Cellular responses to replication-associated DNA damage are centred around Proliferating Cell Nuclear Antigen (PCNA), a DNA clamp that acts as a processivity factor for eukaryotic DNA polymerases. Structurally, ZRANB3 belongs to the Sucrose Non-Fermenting 2 (SNF2) family of ATPases and contains several identifiable domains and motifs, which provide specificity for a number of defined substrates. These include the amino-terminal SNF2 ATPase core, two PCNA binding motifs (the PIP box and the APIM motif), a specific type of zinc-finger (Npl4 Zinc-Finger, NZF) and the HNH nuclease domain (named after the three most conserved residues). We have previously identified ZRANB3 as a structure-specific endonuclease that plays a role in the replication stress response. We further defined PCNA as a key regulator of ZRANB3 function, which recruits ZRANB3 to the sites of stalled DNA replication and stimulates its endonuclease activity.

To gain structural insight into the ZRANB3 HNH domain, we solved the crystal structure of the C-terminal region of the ZRANB3 (residues 948-1067) by experimental phasing. The HNH structure contains two HNH molecules in the asymmetric unit that are structurally similar, with an RMSD of 0.76 Å over 117 equivalent Cα atoms. Each HNH molecule contains one two-stranded anti-parallel β-sheet (β1–β2) surrounded by eight helices (α1–α8). The structure adopts a ββα fold, typically found in the HNH protein family. It also contains a non-catalytic zinc-finger coordinated with four cysteine residues, conserved in a subset of HNH proteins containing the C-x-x-C dyad14. Overlays of the ZRANB3 HNH structure with its closest structural homologues showed that this ZRANB3-specific HNH insert adopts a well-structured α-helical domain. Analysis of the electrostatic surface potential of the HNH domain revealed a predominantly electropositive face, with a continuous positively charged region encompassing helices α1 and α8, as well as helices α2 and α3 in the ZRANB3-specific helical domain. Although the structure of the ZRANB3 HNH domain does not reveal the presence of a divalent cation in the putative active site, residues Asp1020, His1021 and His1045 assume equivalent positions to the catalytically important residues within the ββα-metal fold of T4 endonuclease VII. By analogy with the T4 endonuclease VII structure, we hypothesized the involvement of Asp1020 and His1045 in metal coordination, and the role of His1021 as a general base in nucleophilic attack. Although the mutations did not have a dramatic effect on DNA-dependent ATP hydrolysis, some of them either substantially reduced (N1036A), or completely abrogated (D1020A, H1021A and H1045A) ZRANB3 endonuclease activity. This is consistent with the proposed catalytic roles of Asp1020, His1021 and His1045 in the nucleolytic cleavage of DNA substrate.

>[2x]SMSNNSYLRAKVFETEHGVCQLCNVNAQELFLRLRDAPKSQRKNLLYATWTSKLPLEQLNEMIRNPGEGHFWQVDHIKPVYGGGGQCSLDNLQTLCTVCHKERTARQAKERSQVRRQSLASK> MSAKPQPIAAANWKCNGTTASIEKLVQVFNEHTISHDVQCVVAPTFVHIPLVQAKLRNPKYVISAQNAIAKSGAFTGEVSMPILKDIGVH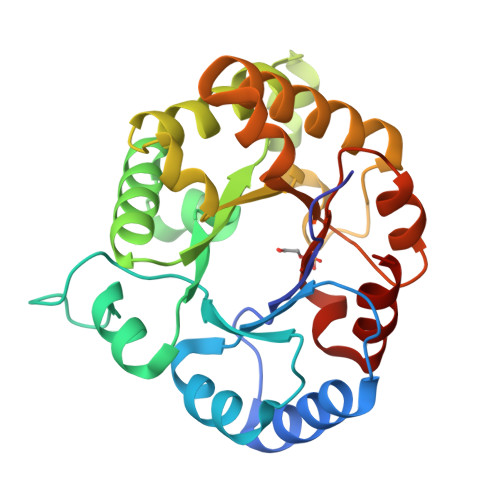WVILGHSERRTYYGETDEIVAQKVSEACKQGFMVIACIGETLQQREANQTAKVVLSQTSAIAAKLTKDAWNQVVLAYEPVWAIGTGKVATPEQAQEVHLLLRKWVSENIGTDVAAKLRILYGGSVNAANAATLYAKPDINGFLVGGASLKPEFRDIIDATR1-[(3~{R})-3-[4-azanyl-3-(4-hydroxyphenyl)pyrazolo[3,4-d]pyrimidin-1-yl]piperidin-1-yl]propan-1-one | C19 H22 N6 O2 | 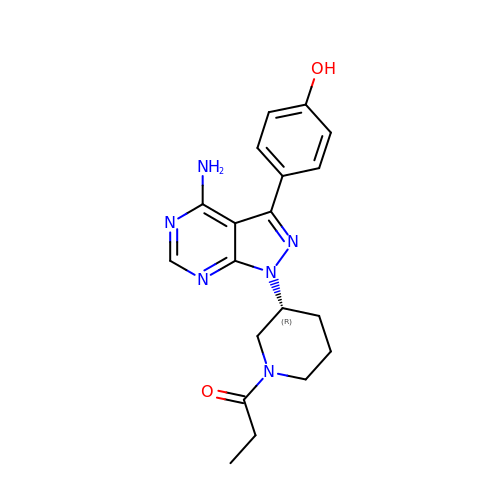OMHARXNEFRLRTL-CYBMUJFWSA-N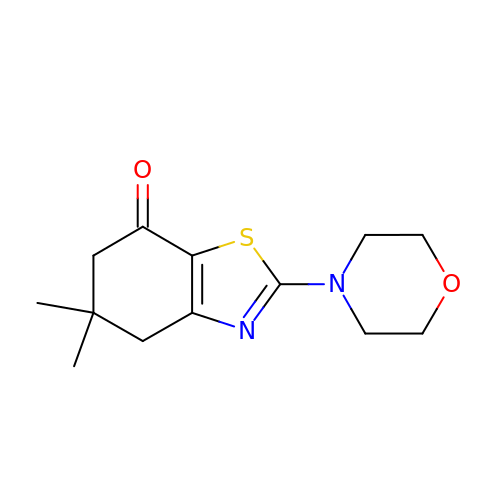5,5-dimethyl-2-morpholin-4-yl-5,6-dihydro-1,3-benzothiazol-7(4H)-one | C13 H18 N2 O2 S | DZXMARZBAUMWLK-UHFFFAOYSA-N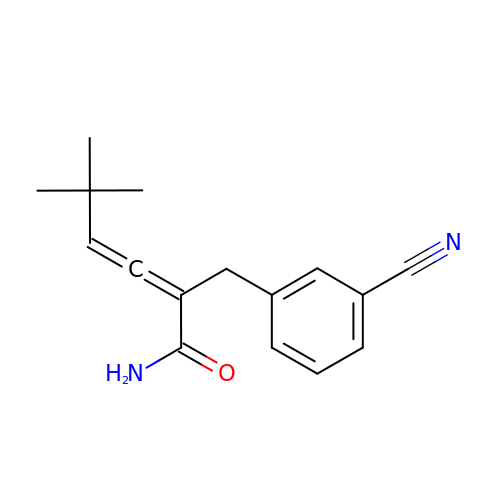2-[(3-cyanophenyl)methyl]-5,5-dimethyl-hexa-2,3-dienamide | C16 H18 N2 O | OISKZRHWMMCOBF-ZETCQYMHSA-N>[2x]MTKKVAIILANEFEDINYSS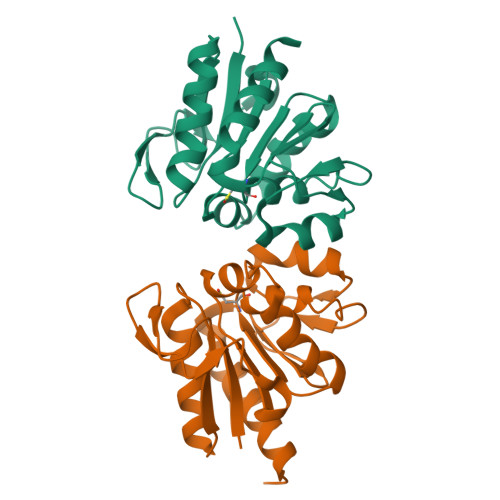PKEALENAGFNTVVIGDTANSEVVGKHGEKVTVDVGIAEAKPEDYDALLIPGGFSPDHLRGDTEGRYGTFAKYFTKNDVPTFAICHGPQILIDTDDLKGRTLTAVLNVRKDLSNAGAHVVDESVVVDNNIVTSRVPDDLDDFNREIVKQLQLEHHHHHH>MEFETIETKKEGNLFWITLNRPDKLNALNAKLLEELDRAVSQAESDPEIRVIIITGKGKAFCAGADITQFNQLTPAEAWKFSKKGREIMDKIEALSKPTIAMINGYALGGGLELALACDIRIAAEEAQLGLPEINLGIYPGYGGTQRLTRVIGKGRALEMMMTGDRIPGKDAEKYGLVNRVVPLANLEQETRKLAEKIAKKSPISLALIKEVVNRGLDSPLLSGLALESVGWGVVFSTEDKKEGVSAFLEKREPTFKGK[6x]

3-HPCD catalyzes the dehydration reaction of 3-hydroxypropionyl-CoA (3-HP-CoA) to produce acryloyl-CoA. The enzyme belongs to the enoyl-CoA hydratase (ECH) family. In the 3-HP sub-pathway, acetyl-CoA is converted to succinyl-CoA by the addition of two molecules of bicarbonate. This sub-pathway consists of nine enzymes, including 3-hydroxypropionyl-CoA dehydratase (3-HPCD). In this study, we report the first crystal structure of 3-HPCD from M. sedula (Ms3HPCD) in complex with CoA, and reveal how the enzyme accommodates 3-HP-CoA as a substrate.

To elucidate the molecular mechanism of Ms3HPCD, we purified, crystallized, and determined its crystal structure at a 1.8 Å resolution. The monomeric structure of Ms3HPCD consists of three distinct domains: One spiral domain and two trimerization domains. The asymmetric unit of the crystal contained six Ms3HPCD monomers, corresponding to a hexameric assembly. The hexamer is formed by dimerization of two trimers. Two glutamate residues (Glu113 and Glu133), which were known to act as catalytic acid and base, respectively, are positioned at the active site of Ms3HPCD. In the vicinity of the catalytic residues, Ala65 and Gly110 are positioned to form an oxyanion hole during enzyme catalysis. In our current structure, the CoA molecule is tightly bound at the substrate binding site, although we did not add the molecule during the protein expression and purification procedure, which enabled us to identify the CoA binding mode of the enzyme. The CoA binding site is formed between three domains, the SD and TD1 of one molecule (Mol I), and the TD2 of the neighboring molecule (Mol II). The pantothenic acid-moiety of CoA is tightly bound and buried in the pocket, whereas the 3′-phosphoadenosine moiety is partially exposed to the surface of Ms3HPCD. Four aromatic residues, such as Phe70, Phe81, Tyr142, and Trp232, play crucial roles in the formation of the unique small size pocket.> GSHMSNVTVSAFTVDKSISEEHVLPSSFIPGSGNIFPKFTSAIPKTAWELWYFDGISKDDKSSIVIGVTRNAEGLKHGGFKVQVFVIWADERTWHRDLFFPESVVSINESGVTDGIWKDATSNSSISFSCAGDLSKASLVFDVPGVVQGDMHLEALPGDTGLDTDARLGPSVYYVRPIGRASVKAQL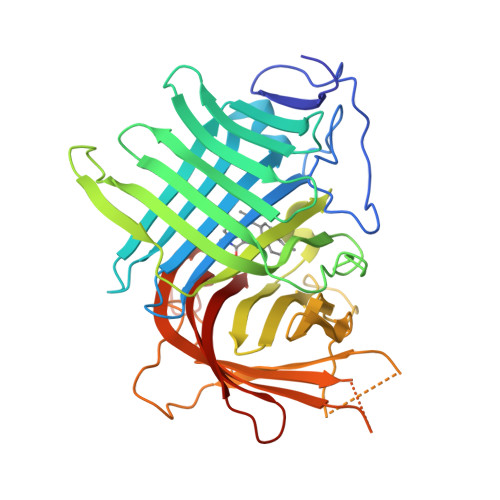SLYSSDATAAEQFSLGTSANGGMDRVWSPLSWPQVMTESYYLRTQVGPYAMQIMRIFPPAGSEDQPSTMARLYREGQLVCVAQHVVTREDALMTHDSLILSKQDNSDSEDVVTGGYRDKNTGYTVEFVEKGNEGQRWKFQVRHERIIWNTPTSRPGPDATGNTGFVEVLCGGTIGESYEGVGTGGQCELS> MRGSHHHHHHGSACELMKPYVLKFQEIRPHSEALVGGKGMNLGACSNIEGVHVPAGFCLTTEAYKRTLAENNEFTQLLQRLSSLKT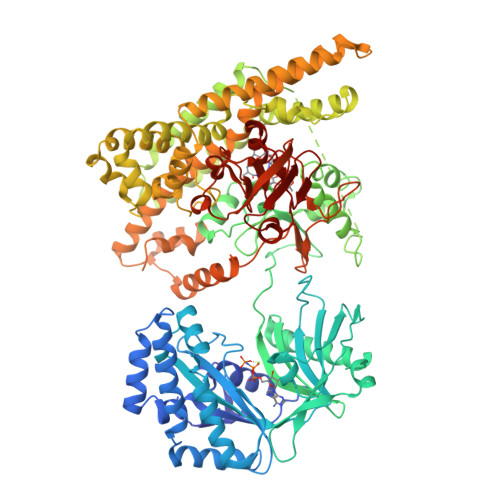SDMDAIREISETIRTLIQHTQIPSEIASYMDATLLDVGGYEMPFAVRSSATAEDLPHASFAGQHDTYLNIIGKDALLQHISMCWASLFTERAIIYRIQNQFDHRKVQLAVVIQQMISPEASGILFTADPITSNRKSLSIDASFGLGEALVSGLVSADSYTVRENTITNKIIATKKLAIYSLKEGGTETRILEKSQQTKQTLTDQQIIQLAKLGRKIEAYFGKPQDIEWCLAEGAFYIVQSRPITTLYPIPEVNEPGNRVYISVAHQQMMTDAMKPLGLSFYLMTTPATMYTAGGRLFVDITQSLSAKVSRDMMVNSLGQSDPLIKDALLTVINKKGFLPPLPTEENPSHATVSGKPPVRSIPDSSSVFELVRNSENSIKHLKQSIETKSGSDLFDFIVEDLEELKRVLFNPTSIDAIMAGMDASAWLNEHIYQWLGEKNVADKLSESAPNNITSQMGLELLDVADVIRPYPAVRAYLEQTKNPDFMNELATLEGGAETKKALEDYLQKYGMRCAGEIDLTKTRWIENPLTLIPLILSNIKNFDSSASMHKFAQGEKEAFHKEQEILRRLQELPDGEQKAMETKEKIDILRHFIGYREYPKYGMINRYFIYKLALLRAGEQLVKDGILQEHEDIYFLYFEELREVVRTGQVDYELINARKRDFATFEKLTPPRILTSDGEMINGEYKRENLPKDAILGLPVSSGTVEGRARVILEMEKADLEDGDILVTAYTDPSWTPAFVSIKGLVTEVGGLMTHGAVIAREYGLPAVVGVENATTIIKDGQQIRINGTEGYIEILD> MLKPILLVEDDKRDLELTLVALERSKLSNEVIVVRDGAQALDYLNREGDFRA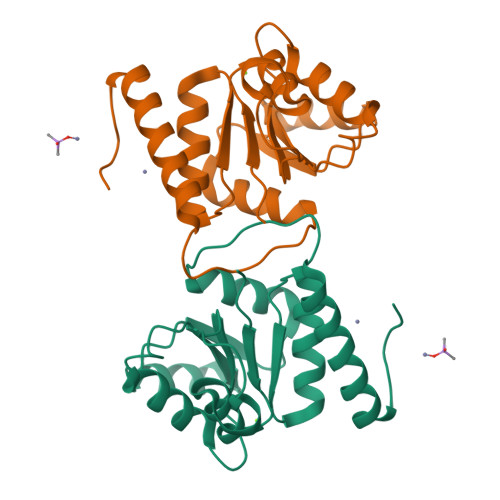REEGNPAVILLDLKLPKVNGLEVLQQVRSSTQLRSIPVVMLTSSQEESDVVKSYELGVNAYVVKPVEFKQFVAAIADLGIFWAVLNEPPPGSMKAMRRYEAKLAAALEHHHHHH> NHTNVKFLFDRSRLLNVIKVLEKDAVFPRPFPTQEGAQQDDGYFCLLTPRPTVASRPATRFGLYANPSGSGVLANTSLDFNFYSLACFTYFRSDLEVTVVSLEPDLEFAVGWFPSGSEYQASSFVYDQLHVPFHFTGRTPRAFASKGGKVSFVLPWNSVSSVLPVRWGGASKLSSATRGLPAHADWGTIYAFVPRPNEKKSTAVKHVAVYIRYKNARAWCPSMLPFRSYK;> GPIPTAPRENSLMFLSTLPDDTVPAYGNVRTPPVNYLPGEITDLLQLARIPTLMAFERVPEPVPASDTYVPYVAVPTQFDDRPLISFPITLSDPVYQNTLVGAISSNFANYRGCIQITLTFCGPMMARGKFLLSYSPPNGTQPQTLSEAMQCTYSIWDIGLNSSWTFVVPYISPSDYRETRAITNSVYSADGWFSLHKLTKITLPPDCPQSPCILFFASAGEDYTLRLPVDCNPSYVF;> WYTGRLNSWTKAVKTFSFQAVPLPGAFLSRQGGLNGGAFTATLHRHFLMKCGWQVQVQCNLTQFHQGALLVAMVPETTLDVKPDGKAKSLQELNEEQWVEMSDDYRTGKNMPFQSLGTYYRPPNWTWGPNFINPYQVTVFPHQILNARTSTSVDINVPYIGETPTQSSETQNSWTLLVMVLVPLDYKEGATTDPEITFSVRPTSPYFNGLRNRYTAG

Seneca Valley virus (SVV) is an oncolytic picornavirus that selectively targets cancer cells by recognizing Tumor endothelial marker 8 (TEM8) as the host receptor. SVV has a typical picornavirus capsid with four capsid proteins; VP1, VP2, and VP3 are characterized by a single jelly roll fold, where eight beta-strands form a barrel-like structure that is distributed at the exterior of the virus, while VP4 is located on the interior of the capsid. The structural architecture consists of four capsid proteins forming a protomer, 5 protomers forming a pentamer, and 12 pentamers assembling into a pseudo T=3 capsid, approximately ~32 nm in diameter. We used cryo-electron microscopy to investigate SVV under acidic conditions and in complex with TEM8 at physiological pH, identifying multiple uncoating intermediates.

We used cryo-EM to image SVV particles after incubation at pH 5 and 37°C with purified TEM8 to explore the structural behavior of SVV. Although the ER-particle from both conditions remains icosahedral, there is a distinct rearrangement of pentamers. Each pentamer has rotated approximately 20° clockwise compared to its position in the F- and A-particles. As a result, the ER-particle is 8% larger than the A-particle and 14% larger than the F-particle, representing a ~44% increase in volume compared to the native state. Similarly, in the ER-particle[C], these include VP1 (S1-S28), VP3 (P61-S66), and VP4. Density corresponding to TEM8 was not visible on the SVV A- and ER-particles under acidic conditions, suggesting that at low pH, the virus potentially loses the affinity for the receptor or binds transiently. A similar SVV ER-particle was identified at pH 6 in the presence of TEM8 (48), which lacked 43 residues at the N-terminus of VP2, whereas our ER-particle at pH 5 lacked 62, indicating the incremental impact of acidification on particle stability. The ER-particle has novel VP2-VP3 and VP3-VP3 contacts at the twofold axis. Overall, the SVV ER-particle is defined by rotated pentamers, an expanded capsid, reduced inter-pentamer contacts, lacks the genome, the VP1 N-terminus, VP2 N-terminus, and the whole of VP4. Our results support this scenario and suggest that our SVV ER-particle may represent a reassociation phenomenon of dissociated pentamers from genome release, as shown for enteroviruses.> VREVCSEQAETGPCRAMISRWYFDVTEGK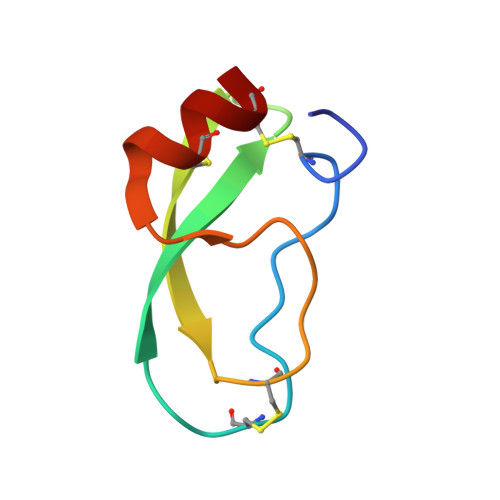CAPFFYGGCGGNRNNFDTEEYCMAVCG>[2x]MSTITLNNGFEMPVIGLGLWRLEKEELRSAILNAIKLGYRHFDAAAHYKTEIDVGNAIAEAIQSGLVKREELFITSKVWNSDHGHVVEACKNSLK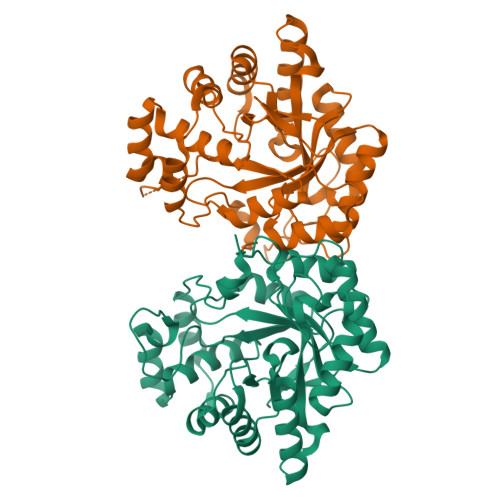KLQLDYLDLYLVHYPLATKHSGVGTTASLLDENKVLDIDVTVSLETTWHDMEKTVSLGLVRSIGLSNYELFLTRDCLSYAKIKPQVSQFETHPYFQRESLVRFCKKHGVVPMAHTPLGGATANVKAFGSISPLEDPVLIGLAKKYQKSVAQIALRWNIERGTPVIPKSSKVERLKENLEVLNFKLEKEDIELINTIDKKFRTTLPSLSWGVDVYA> MEPAAGSSMEPSADWLATAAARGRVEEVRALLEAGANPNAPNSYGRRPIQVMMMGSARVAELLLLHGAEPNCADPATLTRPVHDAAREGFLDTLVVLHRAGARLDVRDAWGRLPVDLAEELGHRDVARYLRAAAGGTRGSNHARIDAAE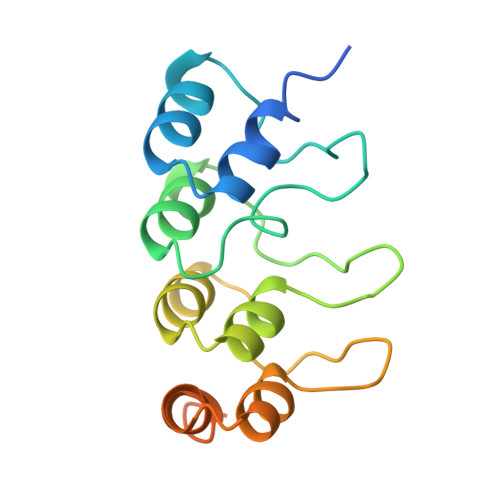GPSDIPD N-((1S,2R)-1-(3-chloro-2-methylphenyl)-1-hydroxypentan-2-yl)-2-oxoindoline-4-carboxamide 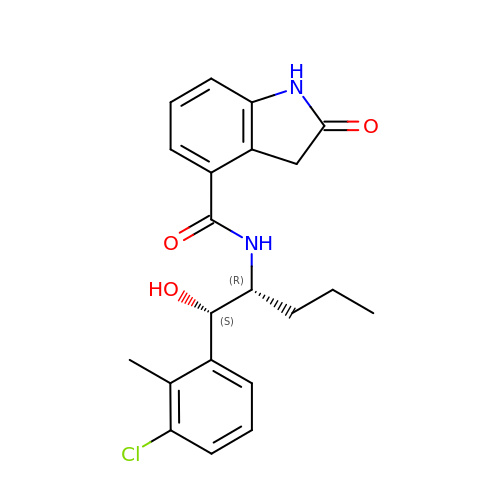| C21 H23 Cl N2 O3 | MQQHOEONXLJMLA-QUCCMNQESA-N(S)-3-{[1-(2-Fluoro-phenyl)-5-hydroxy-1H-pyrazole-3-carbonyl]-amino}-3-o-tolyl-propionic 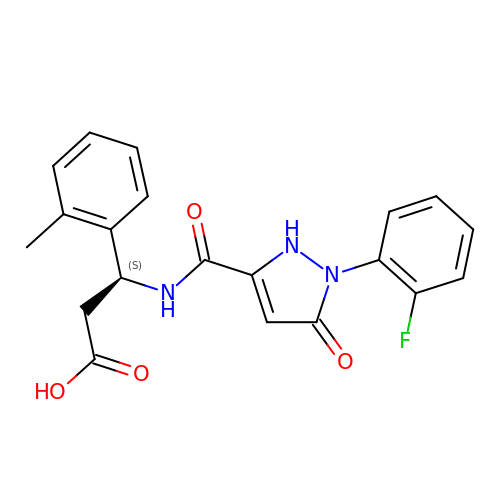acid | C20 H18 F N3 O4 | DGGLFHJMXJUSDG-HNNXBMFYSA-N>MDTPNKDDSIIRF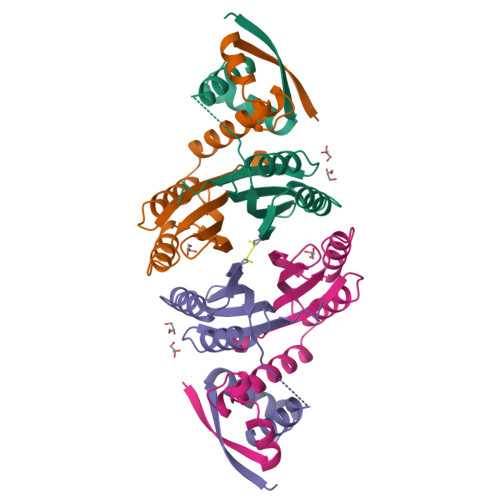SVSLQQNLLDELDNRIIKNGYSSRSELVRDMIREKLVEDNWAEDNPNDESKIAVLVVIYDHHQRELNQRMIDIQHASGTHVLCTTHIHMDEHNCLETIILQGNSFEIQRLQLEIGGLRGVKFAKLTKASSFEYNE[2x]>[4x]MKNQVKKILGMSVVAAMVIVGCSHAPKSGISKSNKAYKEATKGAPDWVVGDLEKVAKYEKYSGVFLGRAEDLITNNDVDYSTNQA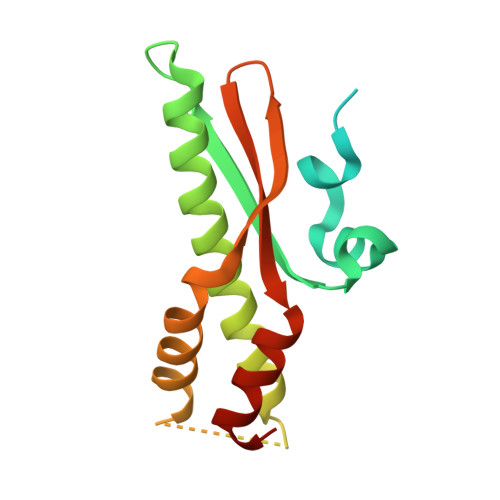TAKARANLAANLKSTLQKDLENEKTRTVDASGKRSISGTDTEKISQLVDKELIASKMLARYVGKDRVFVLVGLDKQIVDKVREELGMVKK>ARQCKAESNTFTGICIAKPPCRQACIREKFT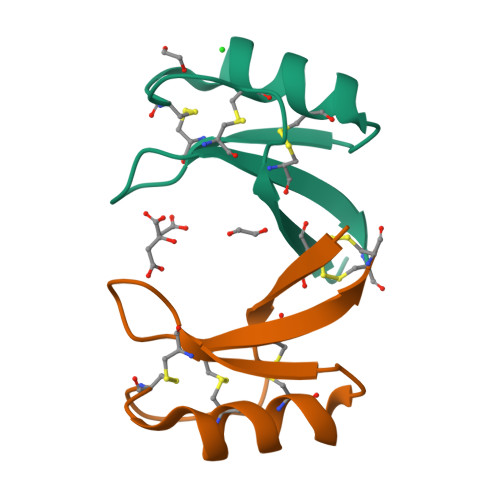DGHCSKVLRRCLCTKRC[12x]>[2x]MRPALYFCGSIRGGREDRTLYERIVSRLRRFGTVLTEHVAAAELGARGEEAAGGDRLIHEQDLEWLQQADVVVAEVTQPSLGVGYELGRAVAFNKRILCLFRPQSGR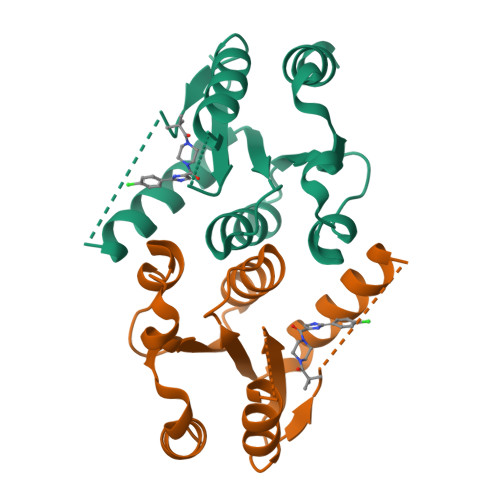VLSAMIRGAADGSRFQVWDYEEGEVEALLDRYFEADPLEENLYFQ> MSLHVTADAPGAAQGGYSVVTFRVPTESETAATTAMTVTLPNVRSARTEPMPGWTARVDRNDKSEAVSVTWTADPGNP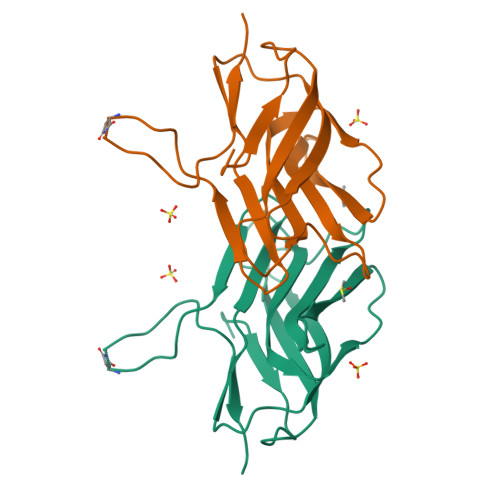GVQPGQFQRFVVSIGPLPSAETVSFPAEQTYSDGRVVAWNQPPAANGSEPEHPAPTLTLATAPGDTEGHHHHHH(2S)-2-hydroxy-2-[2-oxo-2-(phosphonooxy)ethyl]butanedioic acid 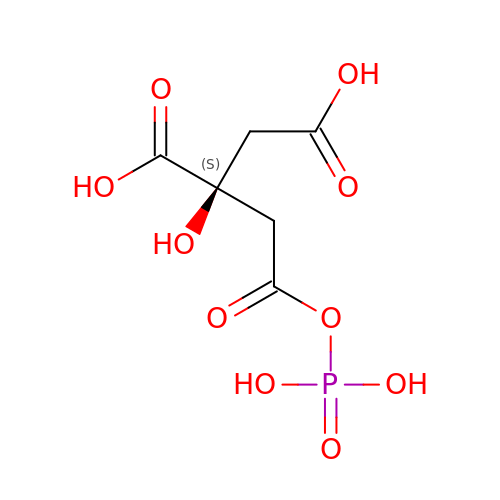| C6 H9 O10 P | RAAPFOXFYNTKEB-LURJTMIESA-N The 2H phosphoesterase superfamily is an ancient group of proteins and protein domains characterized by a common fold and a few conserved active site residues. E. coli LigT is a 20-kDa protein that exhibits 2′,3′-cyclic nucleotide 3′-phosphodiesterase and 2′-5′-ligase/phosphodiesterase activities, but the biological function of the enzyme is unknown. The LigT structure presents a typical 2H phosphoesterase fold, in which the catalytic residues reside at the beginning of strands β2 and β6. As in other 2H family members, the active site has 2-fold symmetry; this symmetry also includes the 4 water molecules at the bottom of the active site, connecting the active-site β strands through water-mediated hydrogen bonds.

The structure of the putative tRNA ligase LigT from E. coli was determined by X-ray crystallography in the apo form. Comparisons to the apo form of the enzyme determined in the current work allow the highlighting of conformational changes and binding determinants of the reactive species. Considering reaction geometry, a water molecule coordinated by His125 in the apo structure can now be designated as the nucleophilic water, analogously to CNPase. In a ligand-free active site, also Phe48 is seen to take a conformation distinct from that seen in ligand complexes. Hence, as opposed to CNPase, in which the active site is to a large extent pre-organized for substrate binding, LigT shows more flexibility.

>GMSEPQRLFFAIDLPAEIREQIIHWRAKHFPPEAGRPVAADNLHLTLAFLGEVSAEKEKALSLLAGRIRQPGFTLTLDDAGQWLRSRVVWLGMRQPPRGLIQLANMLRSQAARSGCFQSNRPFHPHITLLRDASEAVTIPPPGFNWSYAVTEFTLYASSFARGRTRYTPLKRWALTQ[4x]>PADDPGEGPSTGPRGQGDGGRRKKGGWFGKHRGQGGSNPKFENIAEGLRALLARSHVERTTDEGTWVAGVFVYGGSKTSLYNLRRGTALAIPQCRLTPLSRLPFGMAPGPGPQPGPLRESIVCYFMVF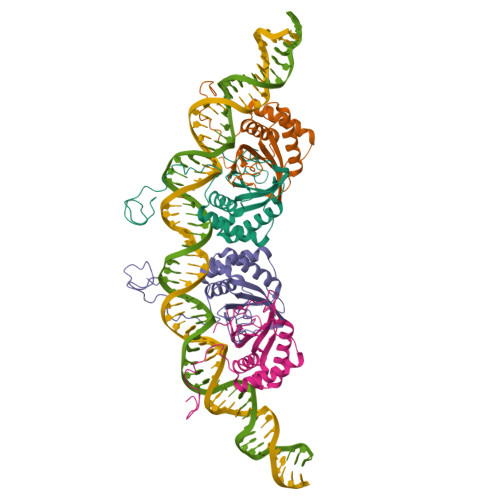LQTHIFAEVLKDAIKDLVMTKPAPTCNIRVTVCSFDDGVDLPPWFPPMVE[4x]> MKIIKDKVAKLSFVALLVTVTAAMFYTPTASAHGEKSQAAFMRMRTIHWFDLNWSKDQVSVNETMSISGKFHVFAGWPETVDKPEVAFLNIGIPGPVFIRAGSWIGGQLVPRSVSLELGETYEFKVLLKARRPGDWHVHTMMNVQGGGPIIGPGKWVTITGSMGDFKNPITTLTGETIDLETYALDGVYGWHLFWYLLGVAWMVYWCRKPVFIPRRIAVDAGKADSLITPTDKKVGMAFAAGTLAIVAVSMGQANEKYPVTTPLQAGLMRGIKSLELPQPTVSVKVVDASYRVPGRAMQMTLEITNNGDSAVRLAEFNTASVRFLDADVYEDDTNYPDDLLAEEGLSVSDNSPLAPGETRTVDVTASDAAWEVYRLADLIYD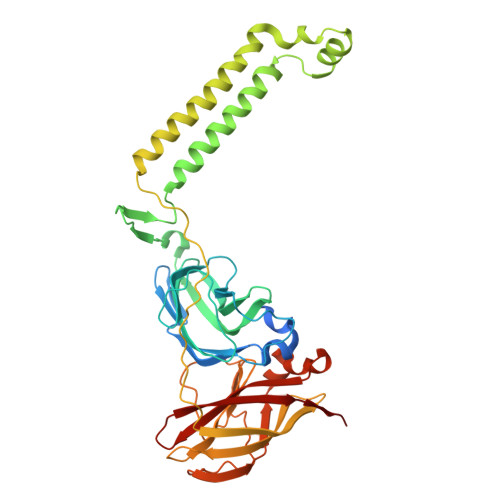PDSRFAGLLFFIDEDGNRQMTMVDAPLIPTFI> GSFTSSGSVNRGPEKIRPECFELLRVLGKGGYGKVFQVRKVTGANTGKIFAMKVLKKAMIVRNAKDTAHTKAERNILEEVKHPFIVDLIYAFQTGGKLYLILEYLSGGELFMQLEREGIFMEDTACFYLAEISMALGHLHQKGIIYRDLKPENIMLNHQGH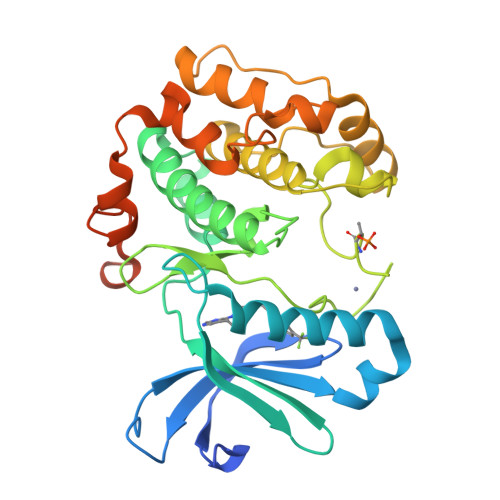VKLTDFGLCKESIHDGTVTHTFCGTIEYMAPEILMRSGHNRAVDWWSLGALMYDMLTGAPPFTGENRKKTIDKILKCKLNLPPYLTQEARDLLKKLLKRNAASRLGAGPGDAGEVQAHPFFRHINWEELLARKVEPPFKPLLQSEEDVSQFDSKFTRQTPVDSPDDST> TTQVKKETITKKEATELVSKVRDLMSQKYTGGSQVGQPIYEIKVGETLSKLKIITNIDELEKLVNALGENKELIVTITDKGHITNSANEVVAEATEKYENSADLSAEANSITEKAKTETNGIYKVADVKASYDSAKDK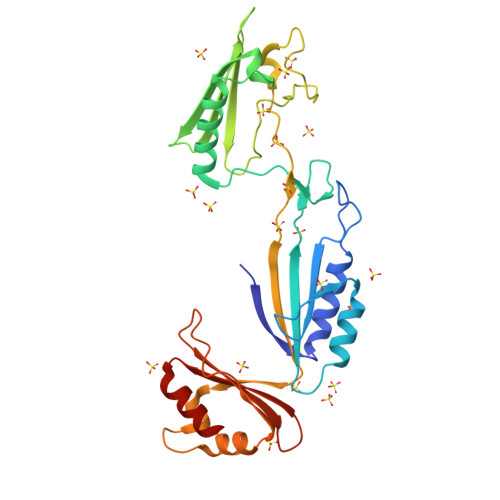LVITLRDKTDTVTSKTIEIGIGDEKIDLTANPVDSTGTNLDPSTEGFRVNKIVKLGVAGAKNIDDVQLAEITIKNSDLNTVSPQDLYDGYRLTVKGNMVANGTSKSISDISSKDSETGKYKFTIKYTDASGKAIELTVESTNEKDLKDAKAALEGNS CD45 is a cell surface phosphatase that shapes the T cell receptor signaling threshold but does not have a known ligand. The primary role of CD45 lies in regulating signal transduction events within immune cells by controlling the phosphorylation status of tyrosine residues on various signaling proteins, such as lymphocyte-specific kinase (Lck). Whereas CD45 contains a large extracellular domain (ECD), it has no known endogenous ligand. A family of adenovirus proteins, including E3/49K, exploit CD45 to evade immunity by binding to the extracellular domain of CD45, suppressing T cell signaling.

We determined the cryo-EM structure of this complex and found that the E3/49K protein is composed of three Ig-domains assembled as “beads on a string” and forces CD45 into a closely abutted dimer by cross-linking the CD45 D3 domain, leading to suppression of its intracellular phosphatase activity. The CD45-E3/49K complex is a 2:1 asymmetric dimer, where two rigid CD45 molecules are positioned in a cis back-to-back orientation and shifted at an approximately 30-degree angle relative to each other. The membrane-proximal regions of two CD45 molecules are in close apposition, likely translating that proximity to its intracellular domains such that the phosphatase domains would be sterically hindered from free access to their substrates. E3/49K uses a “beads on a string” interaction mode with CD45: all three domains of E3/49K protein converge on the CD45 D3 domain, but each uses a different contact surface, resulting in an asymmetric complex. The CD45 D3 domain contains three entirely distinct interaction interfaces with different domains of E3/49K. The E3/49K R1 and R2 domains engage the “front” and R3 with the “back” face of D3 domains in a perpendicular and parallel manner, respectively. The R1 and R2 domains share an overlapping, but molecularly distinct, docking site at the “front” face of CD45 D3 domain with ~ 682-Å and ~ 430-Å of non-polar and ~ 596-Å and ~ 436-Å polar buried surface areas, respectively. However, despite both interfaces centering around residues Arg399 and Ile440 of CD45 D3, they use starkly different detailed modes of engagement. The R1–D3 domain interface of CD45 monomer “a” is mediated by four hydrogen bonds (H-bonds), and many van der Waals (vdW) interactions involving R1 residues Tyr26, Thr28, Gly30, Leu31, Trp32 contacting mostly Arg399 and Thr24, Tyr69, Gly73, Thr74 and Lys76, which contact around Ile440. Strikingly, Lys60 of R1 also forms additional H-bond with the other CD45 D3 domain.

>[2x]QSPTPSPTGLTTAKMPSVPLSSDPLPTHTTAFSPASTFERENDFSETTTSLSPDNTSTQVSPDSLDNASAFNTTGVSSVQTPHLPTHADSQTPSAGTDTQTFSGSAANAKLNPTPGSNAISDVPGERSTASTFPTDPVSPLTTTLSLAHHSSAALPARTSNTTITANTSDAYLNASETTTLSPSGSAVISTTTIATTPSKPTCDEKYANITVDYLYNKETKLFTAKLNVNENVECGNNTCTNNEVHNLTECKNASVSISHNSCTAPDKTLILDVPPGVEKFQLHDCTQVEKADTTICLKWKNIETFTCDTQNITYRFQCGNMIFDNKEIKLENLEPEHEYKCDSEILYNNHKFTNASKIIKTDFGSPGEPQIIFCRSEAAHQGVITWNPPQRSFHNFTLCYIKETEKDCLNLDKNLIKYDLQNLKPYTKYVLSLHAYIIAKVQRNGSAAMCHFTTKSAPPSQVWNMTVSMTSDNSMHVKCRPPRDRNGPHERYHLEVEAGNTLVRNESHKNCDFRVKDLQYSTDYTFKAYFHNGDYPGEPFILHHSTSYNS;> GFHTINATWWANITLVGPPDTPVTWYDTQGLWFCNGSRVKNPQIRHTCNDQNLTLIHVNKTYERTYMGYNRQGTKKEDYKVVVIPPPPATVKPQPEPEYVFVYMGENKTLEGPPGTPVTWFNQDGKKFCEGEKVLHPEFNHTCDKQNLILLFVNFTHDGAYLGYNHQGTQRTHYEVTVLDLFPDSGQMKIENHSEETEQKNDEHHNWQKQGGQKQGGQKTNQTKVNDRRKTAQKRPSKLKPATIEAMLVTVTAGSNLTLVGPKAEGKVTWFDGDLKRPCEPNYRLRHECNNQNLTLINVTKDYEGTYYGTNDKDEGKRYRVKVNTTNSQSVKIQGAPHHHHHH> GASCEKDPDMGKLDDNYLVYTNYDKQANFKDFSTFYLADKILVISDSKEPEYLEGEGAEQILAAYTENMEAKGYQPAADKESADLGIQVSYIASTYYFTGYTQPEWWWGYPGYWGPSYWGNWGGWYYPYAVTYSY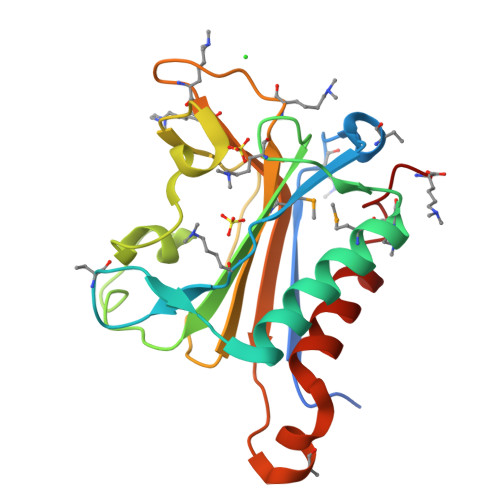STNSFITEMVNLKADEGEGKKLPVVWTSYLTGFETGSKAINRTLAIEAVNQSFTQSPYLTNK Human cytomegalovirus (HCMV) causes congenital disease with long-term morbidity. HCMV glycoprotein B (gB) transitions irreversibly from a metastable prefusion to a stable postfusion conformation to fuse the viral envelope with a host cell membrane during entry. Antibodies directed against the viral fusogen, glycoprotein B (gB), can neutralize HCMV.

We stabilized prefusion gB on the virion with a fusion inhibitor and a chemical cross-linker, extracted and purified it, and then determined its structure to 3.6-Å resolution by electron cryomicroscopy. The molecular model of prefusion gB fits well in the low-resolution electron cryo-ET envelope of prefusion gB on the virion, confirming that the structure represents a prefusion conformation and that the stabilization of the prefusion gB by the fusion inhibitor and chemical cross-linker did not substantially distort its overall structure. In the model, prefusion gB forms a tripod that is approximately 100 Å in diameter and extends 110 Å above the viral membrane. The central core of the ectodomain is formed by three trimeric coiled coils centered on the threefold axis with an N- to C-terminal polarity toward the center of the virion: one membrane distal in domain III (α3, yellow), one membrane proximal in domain V (α7, red), and the TM domain, which is embedded in the viral envelope (α10, olive). The legs of the prefusion trimer are formed by the peripheral, globular domain I of each protomer, which has the fusion loops at its membrane-proximal tip (blue). In the prefusion conformation, domain V residues 639 to 669 from each protomer are sandwiched between domains I and IV of an adjacent protomer, “tacking” domain I down to the central core. Domain I is further constrained by the interaction of multiple aromatic side chains (Y153, Y155, Y160, W240, and Y242) in its two fusion loops (between β3 and β4 and between β9 and β10) with the amphipathic α8 and α9 helices of an adjacent protomer’s MPR, which forms a “scabbard,” shielding the hydrophobic tip of domain I until it is unsheathed to insert into a host cell membrane in the extended intermediate. The interactions between WAY-174865 and gB are mainly hydrophobic and aromatic, involving multiple hydrophobic residues, including Y153 and Y155 in the fusion loop; L712, L715, I730, A738, and F747 in the MPR; and P751 and F752 in the TM. HCMV strain AD169 escapes inhibition through mutation of residues homologous to strain Towne G734 and F752 (18), which are WAY-174865 binding residues on α9 of the MPR and α10 of the TM, respectively. The visualization of a fusion inhibitor bound in the interface between the fusion loops, MPRs, and proximal TM domain shows how the inhibitor stabilizes the prefusion conformation and provides high-resolution data that can guide structure-based drug design.

>[3x]MESRIWCLVVCVNLCIVCLGAAVSSSSTRGTSATHSHHSSHTTSAAHSRSGSVSQRVTSSQTVSHGVNETIYNTTLKYGDVVGVNTTKYPYRVCSMAQGTDLIRFERNIVCTSMKPINEDLDEGIMVVYKRNIVAHTFKVRVYQKVLTFRRSYAYIHTTYLLGSNTEYVAPPMWEIHHINSHSQCYSSYSRVIAGTVFVAYHRDSYENKTMQLMPDDYSNTHSTRYVTVKDQWHSRGSTWLYRETCNLNCMVTITTARSKYPYHFFATSTGDVVDISPFYNGTNRNASYFGENADKFFIFPNYTIVSDFGRPNSALETHRLVAFLERADSVISWDIQDEKNVTCQLTFWEASERTIRSEAEDSYHFSSAKMTATFLSKKQEVNMSDSALDCVRDEAINKLQQIFNTSYNQTYEKYGNVSVFETTGGLVVFWQGIKQKSLVELERLANRSSLNLTHNRTKRSTDGNNATHLSNMESVHNLVYAQLQFTYDTLRGYINRALAQIAEAWCVDQRRTLEVFKELSKINPSAILSAIYNKPIAARFMGDVLGLASCVTINQTSVKVLRDMNVKESPGRCYSRPVVIFNFANSSYVQYGQLGEDNEILLGNHRTEECQLPSLKIFIAGNSAYEYVDYLFKRMIDLSSISTVDSMIALDIDPLENTDFRVLELYSQKELRSSNVFDLEEIMREFNSYKQRVKYVEDKVVDPLPPYLKGLDDLMSGLGAAGKAVGVAIGAVGGAVASVVEGVATFLKNPFGAFTIILVAIAVVIIIYLIYTRQRRLCMQPLQNLFPYLVSADGTTVTSGNTKDTSLQAPPSYEESVYNSGRKGPGPPSSDASTAAPPYTNEQAYQMLLALVRLDAEQRAQQNGTDSLDGQTGTQDKGQKPNLLDRLRHRKNGYRHLKDSDEEENV> MGSSKPLKGFVICCTSIDLKQRTEISTKATKLGAAYRSDFTKDVTHLIAGDF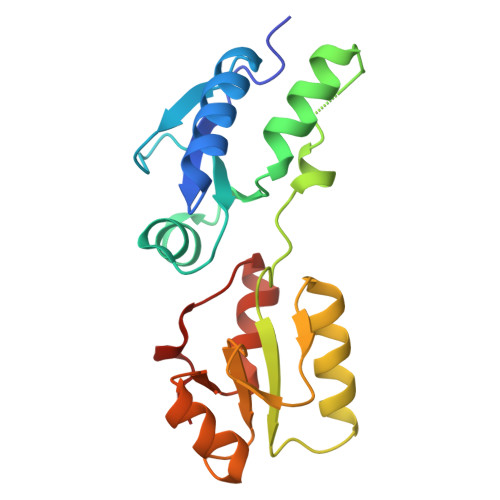DTPKYKFAAKSRPDIKIMSSEWIPVLYESWVQGEDLDDGLLVDKHLLPTLFKCRVCLTNIGQPERSRIENYVLKHGGTFCPDLTRDVTHLIAGTSSGRKYEYALKWKINVVCVEWLWQSIQRNAVLEPQYFQLD>[2x]SMSSAIKSYKSVLRPNERKNQLLKSTIQCLEDGSAFFFKMLQGLFGGITPEIVRFSTEQEKQQQDIALWCAVNWFRPVSQDSLTHTIASDNLVEKFEEYYGGTASDAIKQYFSASIGESYYWNDCRQQYYDLCRELGVEVSDLTHDLEILCREKCLAVATESNQNNSIISVLFGTGEKEDRSVKLRITKKILEAISNLKEIPKNVAPIQEIILNVAKATKETFRQVYAGNLGAPSTLEKFIAKDGQKEFDLKKLQTDLKKVIRGKSKERDWCCQEELRSYVEQNTIQYDLWAWGEMFNKAHTALKIKSTRNYNFAKQRLEQFKEIQSLNNLLVVKKLNDFFDSEFFSGEETYTICVHHLGGKDLSKLYKAWEDDPADPENAIVVLCDDLKNNFKKEPIRNILRYIFTIRQECSAQDILAAAKYNQQLDRYKSQKANPSVLGNQGFTWTNAVILPEKAQRNDRPNSLDLRIWLYLKLRHPDGRWKKHHIPFYDTRFFQEIYAAGNSPVDTCQFRTPRFGYHLPKLTDQTAIRVNKKHVKAAKTEARIRLAIQQGTLPVSNLKITEISATINSKGQVRIPVKFDVGRQKGTLQIGDRFCGYDQNQTASHAYSLWEVVKEGQYHKELGCFVRFISSGDIVSITENRGNQFDQLSYEGLAYPQYADWRKKASKFVSLWQITKKNKKKEIVTVEAKEKFDAICKYQPRLYKFNKEYAYLLRDIVRGKSLVELQQIRQEIFRFIEQDCGVTRLGSLSLSTLETVKAVKGIIYSYFSTALNASKNNPISDEQRKEFDPELFALLEKLELIRTRKKKQKVERIANSLIQTCLENNIKFIRGEGDLSTTNNATKKKANSRSMDWLARGVFNKIRQLAPMHNITLFGCGSLYTSHQDPLVHRNPDKAMKCRWAAIPVKDIGDWVLRKLSQNLRAKNIGTGEYYHQGVKEFLSHYELQDLEEELLKWRSDRKSNIPCWVLQNRLAEKLGNKEAVVYIPVRGGRIYFATHKVATGAVSIVFDQKQVWVCNADHVAAANIALTVKGIGEQSSDEENPDGSRIKLQLTS

Two Cas12i (Cas12i1 and Cas12i2) proteins have crRNA-guided dsDNA cleavage activity. In addition to the double-strand DNA (dsDNA) cleavage activity, Cas12i2 cleaves ssDNA in trans upon crRNA forming heteroduplex with the complementary ssDNA, as well as processes the pre-crRNA to form the mature crRNA. The Cas12i2 consists of the recognition (REC) and nuclease (NUC) lobes connected by the wedge (WED) domain. The RuvC domain is the sole DNase catalytic domain in Cas12i2, with catalytic residues Asp599, Glu833, and Asp1019 lining the active pocket.

In contrast to the DNA-bound Cas12i2 ternary complex, in which 26 nucleotides within the crRNA spacer are traceable, the spacer region is mostly disordered in the binary complex. Only 4 nucleotides in the seed region, 6 nucleotides in the central area and 9 nucleotides at the 3′-ends of the spacer were observed in the binary complex, suggesting the crRNA seed region is only partially pre-ordered. In addition, the PI domain is almost completely disordered in the Cas12i2–crRNA binary complex, while it is ordered in all DNA-bound Cas12i2 ternary complexes, suggesting that the PI domain is not pre-ordered prior to DNA binding and is stabilized by interactions with the PAM sequence. Comparison of the binary and ternary complexes shows that the Helical-II domain is ordered in both the Cas12i2–crRNA binary and the fully paired DNA-bound Cas12i2 ternary complexes, while it is flexible in the partially paired DNA-bound complexes, suggesting that the base-pairing in the seed region increases the flexibly of the Helical-II domain. In the Cas12i2–crRNA binary complex, the Helical-II domain that is positioned closed to the RuvC domain acts like a lid covering and closing off the RuvC catalytic pocket. In addition, the loop (residues 386–393) within the Helical-II domain inserts into the RuvC catalytic pocket, occupying the substrate ssDNA binding position. Therefore, the Helical-II domain blocks the active site of the RuvC domain prior to the target DNA binding. Thus, RuvC catalytic pocket is inactive prior to formation of the guide:target heteroduplex, which induces a rearrangement of the Helical-II domain and activates the RuvC catalytic pocket.>[2x]MATNA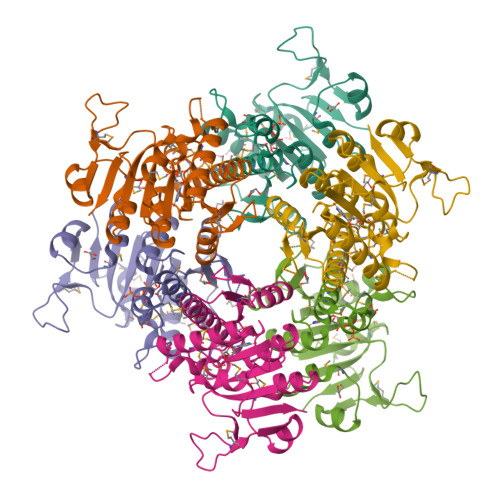KPVYKRILLKLSGEALQGTEGFGIDASILDRMAQEIKELVELGIQVGVVIGGGNLFRGAGLAKAGMNRVVGDHMGMLATVMNGLAMRDALHRAYVNARLMSAIPLNGVCDSYSWAEAISLLRNNRVVILSAGTGNPFFTTDSAACLRGIEIEANVVLKATKVDGVFTADPAKDPTATMYEQLTYSEVLEKELKVMDLAAFTLARDHKLPIRVFNMNKPGALRRVVMGEKEGTLITE> QIRYSVPEETDKGTVVGNISKDLGLEPRELAERGVRIVSRGR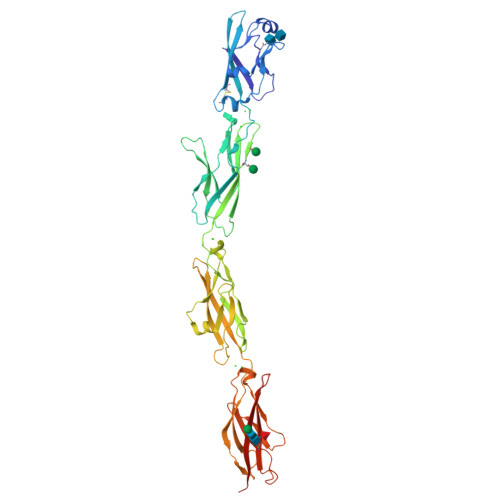SQLFSLNPRGGSLVTAGRIDREELCAQSTPCLVNINILVEEKGKLFGVEIEITDINDNNPKFHVGDLEVKINEIAAPGARYPLPEAVDPDVGINSLQSYQLSPNRHFSLHLQTGDDGTINPELVLERTLDREEEPTHHLVLTASDGGEPRRSSTALIQITVLDTNDNAPVFDQPVYRVKVLENVAPGTLLLTVRASDPDEGVNGKVTYKFRKINEKQSLLFHLHENTGEMTVAKNLDYEECSLYEMEIQAEDVGALLGRSKVIIMVEDVNDNRPEVTITSLFNPVLENSLPGTVIAFLNVHDQDSGKNGQVVCYTHDNLPFKLEKSIDNYYRLVTWKYLDREKVSTYNITVIASDLGAPPLSTETYIALTVADTNDHHHHHHHH>[4x]IREILKMGDERLLRIAQPVPSELLGSEELQRLIDDMFETMHHVGGVGLAAPQIGVDLQLVIFGFERSERYPDAPAVPPTILLN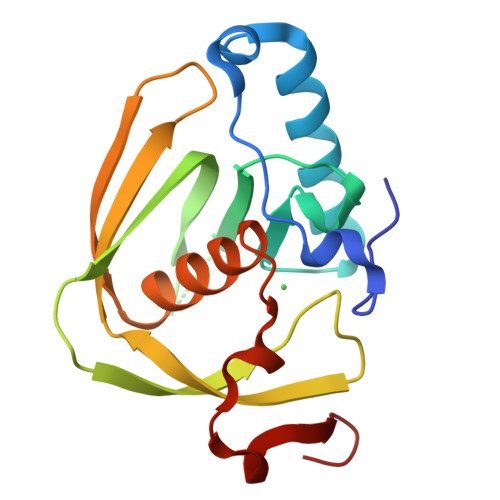PRITPLDDEMEEGWEGCLSVPGLRGAVSRHRRIRYQGLDPQGQPIDRSVEGFHARVVQHECDHLIGRLYPSRITDFSKFGFTEVL> TENILRKSDEEIQKEITARVKALESMLIEQGILTTSMIDRMAEIYENEVGPHLGAKVVVKAWTDPEFKKRLLADGTEACKELGIGGLQGEDMMWVENTDEVHHVVVCSLCSCYPWPVLGLPPNWFKEPQYRSRVVREPRQLLKEEFGFEVPPSKEIKVWDSSSEMRFVVLPQRPAGTDGWSEEELATLVTRESMIGVEPAKAV;> MNGVYDVGGTDGLGPINRPADEPVFRAEWEKVAFAMFPATFRAGFMGLDEFRFGIEQMNPAEYLESPYYWHWIRTYIHHGVRTGKIDLEELERRTQYYRENPDAPLPEHEQKPELIEFVNQAVYGGLPASREVDRPPKFKEGDVVRFSTASPKGHARRARYVRGKTGTVVKHHGAYIYPDT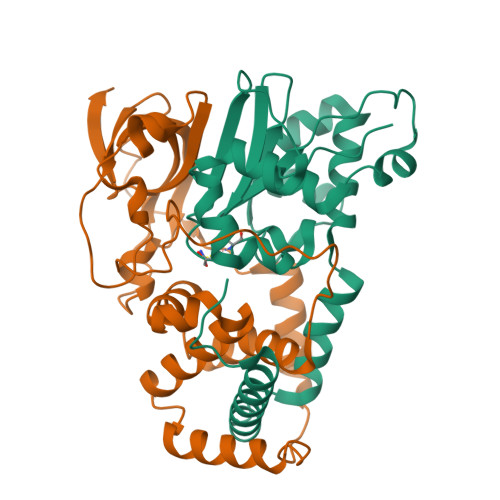AGNGLGECPEHLYTVRFTAQELWGPEGDPNSSVYYDCWEPYIELVDT(3~{S})-3-[[(1~{S},3~{S})-3-methylcyclohexyl]methyl]-6,8-bis(oxidanyl)-3,4-dihydro-2~{H}-isoquinolin-1-one 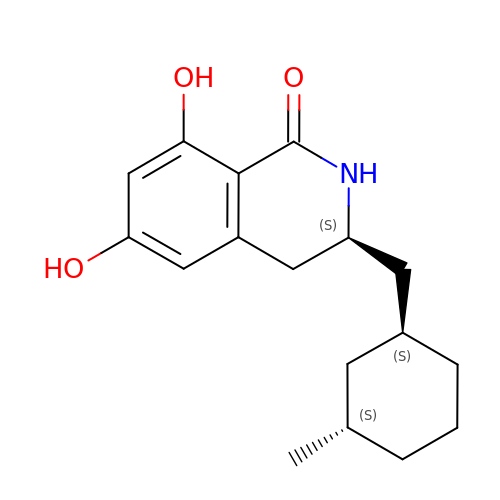| C17 H23 N O3 | YKYWGEWGZHSEGR-GVXVVHGQSA-N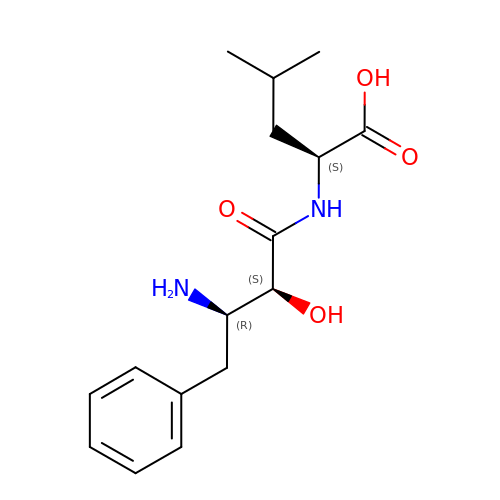2-(3-AMINO-2-HYDROXY-4-PHENYL-BUTYRYLAMINO)-4-METHYL-PENTANOIC ACID | C16 H24 N2 O4 | VGGGPCQERPFHOB-RDBSUJKOSA-N> MGHHHHHHAMEGKITPVSVKKVDDKVTLYKTTATADSDKFKISQILTFNFIKDKSYDKDTLVLKATGNINSGFVKPNPNDYDFSKLYWGAKYNVSISSQSNDS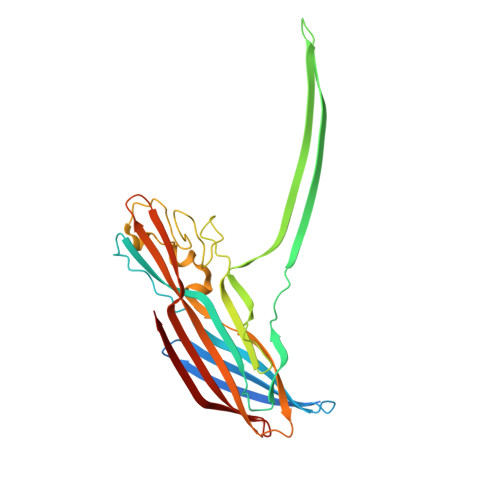VNVVDYAPKNQNEEFQVQNTLGYTFGGDISISNGLSGGLNGNTAFSETINYKQESYRTTLSRNTNYKNVGWGVEAHKIMNNGWGPYGRDSFHPTYGNELFLAGRQSSAYAGQNFIAQHQMPLLSRSNFNPEFLSVLSHRQDGAKKSKITVTYQREMDLYQICWNGFYWAGANYKNFKTRTFKSTYEIDWENHKVKLLDTKETENNK>[2x]MQDNMMWWRGGVIYQIYPRSFLDSRGDGVGDLNGITEKLDYVASLNVDGIWLSPFFTSPMLDFGYDVSDYRDVDPMFGTLEDFKALLEKAHSLGLKVMIDQVISHTSDQHPWFQESRQN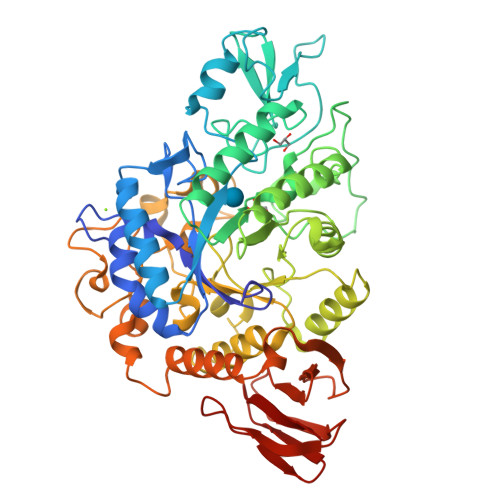RTNPKADWFVWADPKPDGTPPNNWLSIFGGSAWTFDSRRQQYYLHNFLTSQPDVNFHHPEARQAQLDNMRFWLDLGVDGFRLNTVNFYFHDAELRDNPPVPKGEAKTLGAPEANPYTWQRHVYDLSRPENLDFLKDLRALMDEYPGTTTVGEIGDDNPLERMAEYTAGGDKLHMAYTFDLLNMPHSASYLREVIERFQRLAGDAWPCWATSNHDVVRSATRWGADEDPHAYPKVMLAVLFSLRGSVCLYQGEELGLPEADVPFERIQDPYGKVLWPEFKGRDGCRTPMPWTDGEQGGFSPVEPWLPMEARHLELAVSRQQDDPNATLNTVRALLAFRRSHPALFDGDLSLVDVGDDLLGFTRQKGDETLLCVFNLTGQEQQTTLPVEVASDLPVAHFTATRDGSTLTLPAYQAAFMQVA>GAMDPSSPNYDKWEMERTDITMKHKLGGGQYGEVYEGVWKKYSLTVAVKTLKEDTMEV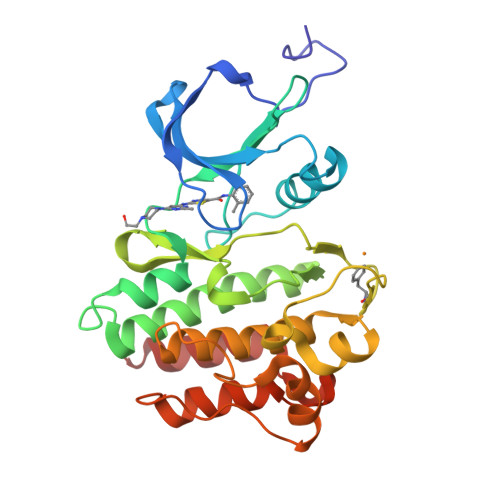EEFLKEAAVMKEIKHPNLVQLLGVCTREPPFYIITEFMTYGNLLDYLRECNRQEVNAVVLLYMATQISSAMEYLEKKNFIHRDLAARNCLVGENHLVKVADFGLSRLMTGDTYTAHAGAKFPIKWTAPESLAYNKFSIKSDVWAFGVLLWEIATYGMSPYPGIDLSQVYELLEKDYRMERPEGCPEKVYELMRACWQWNPSDRPSFAEIHQAFETMFQES[2x]> MPEGADPVAEVKTALAGFLKEVKGFQDDVKTRLQQQEERVTMLQTKTYAGRHALAAAATEEAPHQKAFAAYLRTGDDDGLRGLSLEGKALNSAVAAEGGYLVDPQTSETIRGVLRSTASLRQIASVVNVEATSFDVLVDKTDMGSGWASETAALSETATPQIDRITIPLHELAAMPKASQRLLDDSAFDIETWLANRIADKFARAEAAAFISGDGVDKPTGFLTKTKVANGAWAWGSLGYVATGAAGDFAAVNASDAVVDLVYALGAEYRANASFVMNSKTAGAVRKMKDADGRFLWADSLAAGEPARLMGYPVLIAEDMPDIAANAYAIAFGDFGNGYTIAERPDLRVLRDPFSA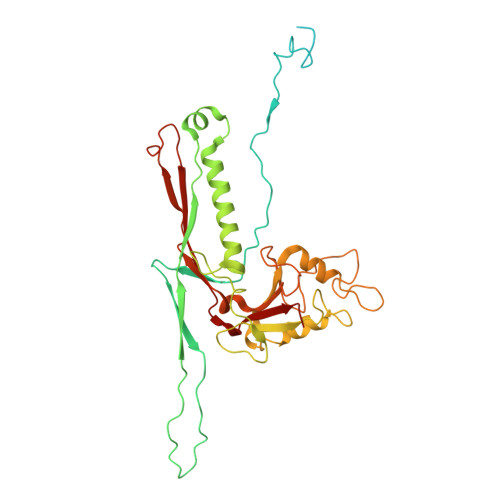KPHVLFYASKRVGGDVSDFAAIKLLKFAA>[2x]VPTTVDFDTLCPEPIFQDRWVATPRGRVFTRTWETSHLRSDVPIVLLHDSLGCVDLWRSFPAALCAATQRRVIAYDRLGFGRSDACLTPPLLSFIDDEPSTSFAALQSAFQLTHFIALGHSVGGCMAVHCAGQYVEQCQGLITIAAQAVNEPRTQQGIEEARAAFQMPEQFAKLEKYHGN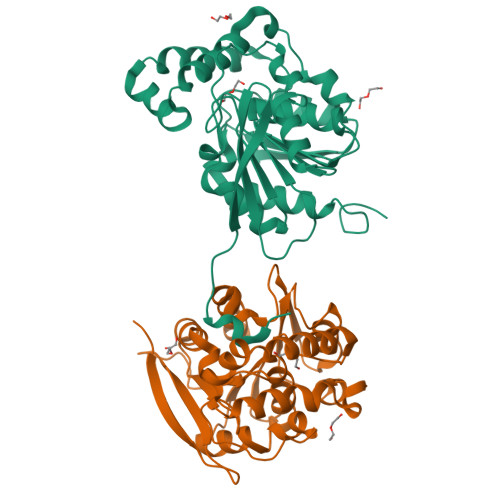KARWVLNGWIDTWLHPAFEHWSLTPALQHVHCPTLVLHGENDEYGSHRQPEGIARHTRGPAHTEILPGVGHVPHREVEAVVVHYVSEFIERLTPGTPGAPA> XAEIAAIEYEQAAIKEEIAAIKDKIAAIKEYIAAIX;> XEKIAAIKEEQAAIEEEIQAIKEEIAAIKYLIAQIX;> XAEIAAIKYKQAAIKNEIAAIKQEIAAIEQMIAAI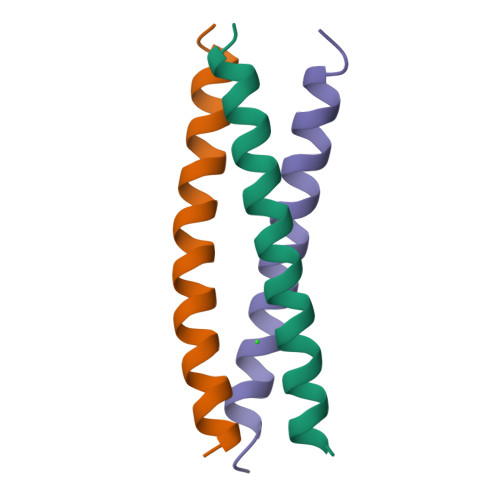X> SNAMADVAESQENAPAERAELTVPEMRQWLRNWVGKAVGK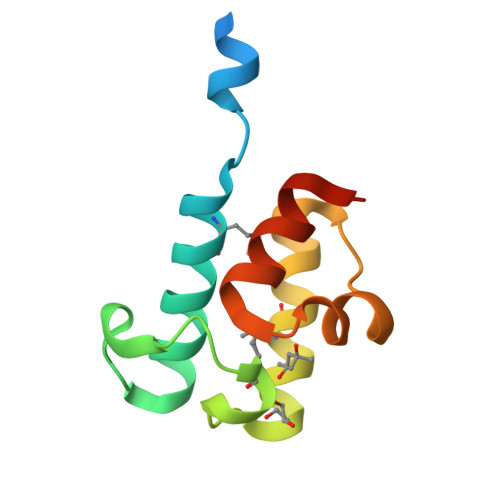APDSIDESVPMVELGLSSRDAVAMAADIEDLTGVTLSVAVAFAHPTIESLATRIIEGEPETDL> GSVFINVKC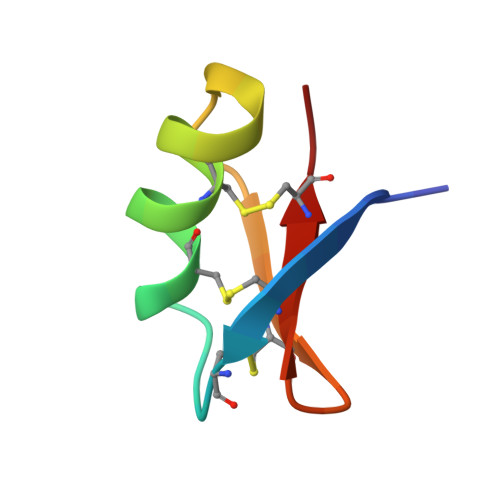RGSPECLPKCKEAIGKSAGKCMNGKCKCYP>NSELDRLSKDDRNWVMQTKDYSATHFSRLTEINSHNVKNLKVAWTLSTGTLHGHEGAPLVVDGIMYIHTPFPNNVYAVDLNDTRKMLWQYKPKQNPAARAVACCDVVNRGLAYVPAGEHGPAKIFLNQLDGHIVALNAKTGEEIWKMENSDIAMGSTLTGAPFVVKDKVLVGSAGAELGVRGYVTAYNIKDGKQEWRAYATGPDEDLLLDKDFNKDNPHYGQFGLGLSTWEGDAWKIGGGTNWGWYAYDPKLDMIYYGSGNPAPWNETMRPGDNKWTMTIWGRDADTGRAKFGYQKTPHDEWDYAGVNYMGLSEQEVDGKLTPLLTHPDRNGLVYTLNRETGALVNAFKIDDTVNWVKKVDLKTGLPIRDPEYSTRMDHNAKGICPSAMGYHNQGIESYDPDKKLFFMGVNHICMDWEPFMLPYRAGQFFVGATLNMYPGPKGMLGQVKAMNAVTGKMEWEVPEKFAVWGGTLATAGDLVFYGTLDGFIKARDTRTGELKWQFQLPSGVIGHPITYQHNGKQYIAIYSGVGGWPGVGLVFDLKDPTAGLGAVGAFRELAHYTQMGGSVFVFSL[8x];>[8x]YDGTHCKAPGNCWEPKPGYPDKVAGSKYDPKHDPNELNKQAESIKAMEARNQKR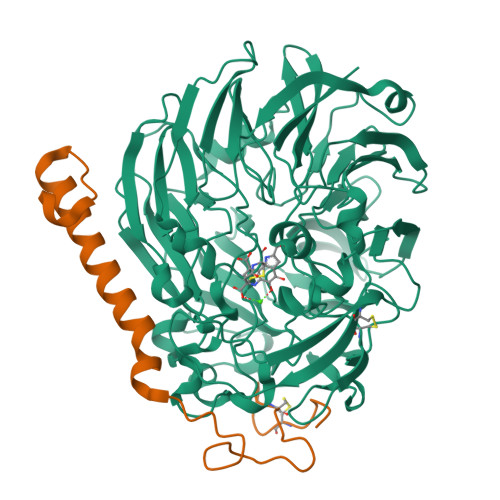VENYAKTGKFVYKVEDIK> MRSRLVGKSLASLYVRPPVTCYTDACEAPVAMWNGAIPLKEVRVMQKGVPVRYVTKLYSHPLEASPTRLSFNDINSMYCVGNDELMQFFPEGLGGKVMQLMPPGHPRGFLYRKEAHLLNLFIDKIQHWQAKRNVLSSLTNNRPGFIIDGPKGCGKSALMCQVVHYARSRNLLTLYVPNAKEWTHGEWCWPSTILPGFFDAPDAARFFLRYFAKANRSTLLSWRLKCTPNDLPVEQGERQPQNLYELCEWGHQVVAP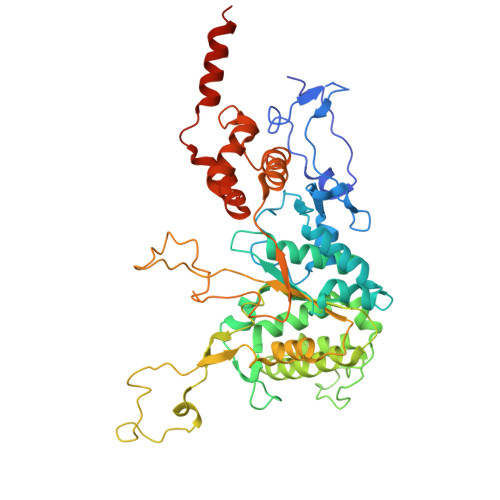ASIDRQSVCVKFLMDELSAEKKLPIVIVVDGWNLFSHDTHFRYPHPDFLRTLASLNDDSTDIDLYPQELPRIPASRLGFVRGLNKMILSKDEPNKFFFTCTTRDFKPFDGISGFPDVETDRFTNSLDEYAPYDAEKDSLFHPIQLGNFDEYEFRAFTRFLVNSGELAGLGWGPLWHFSSDFERKLYKIGFLSNRNPQGVIDHYHQELVWRYEYQRTRQKQYLLHRNMELVVSKRKNRHAEPKGG CYCLODODECYL 3,4,6-TRIDEOXY-3-(DIMETHYLAMINO)-BETA-D-XYLO-HEXOPYRANOSIDE | C20 H39 N O3 | 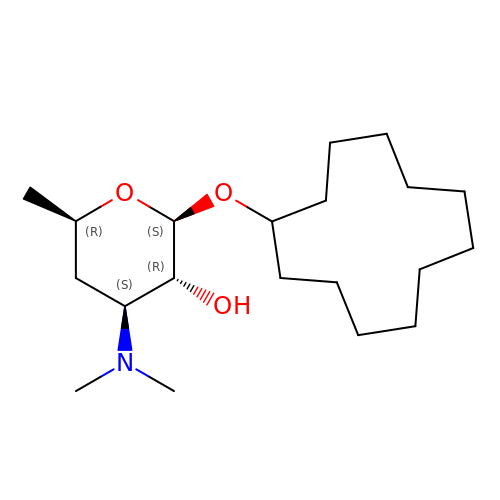KZKWNNFETLOBHX-MDNKFWRPSA-N> IVGGYTCAANSVPYQVSLNSGSHFCGGSLINSQW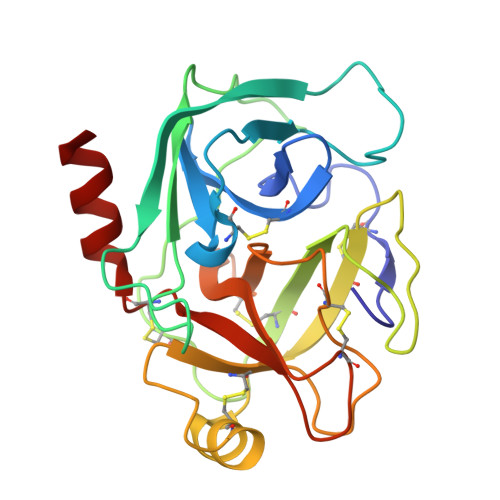VVSAAHCYKSRIQVRLGEHNIDVLEGNEQFINAAKIITHPNFNGNTLDNDIMLIKLSSPATLNSRVATVSLPRSCAAAGTECLISGWGNTKSSGSSYPSLLQCLKAPVLSDSSCKSAYPGQITGNMICVGFLEGGKDSCQGDSGGPVVCNGQLQGIVSWGYGCAQKNKPGVYTKVCNYVNWIQQTIAAN> MSEMTPREIVSELDKHIIGQDNAKRSVAIALRNRWRRMQLNEELRHEVTPKNILMIGPTGVGKTEIARRLAKLANAPFIKVEATKFTEVGY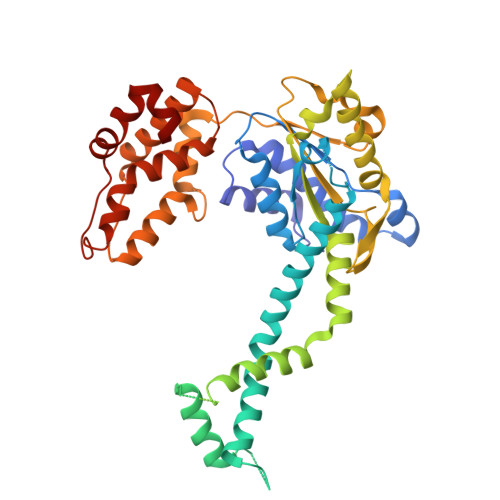VGKEVDSIIRDLTDAAVKMVRVQAIEKNRYRAEELAEERILDVLIPPAKNNWGQTEQQQEPSAARQAFRKKLREGQLDDKEIEIDLAAAPMGVEIMAPPGMEEMTSQLQSMFQNLGGQKQKARKLKIKDAMKLLIEEEAAKLVNPEELKQDAIDAVEQHGIVFIDEIDKICKRGESSGPDVSREGVQRDLLPLVEGCTVSTKHGMVKTDHILFIASGAFQIAKPSDLIPELQGRLPIRVELQALTTSDFERILTEPNASITVQYKALMATEGVNIEFTDSGIKRIAEAAWQVNESTENIGARRLHTVLERLMEEISYDASDLSGQNITIDADYVSKHLDALVADEDLSRFIL>[12x]MGSSHHHHHHSQDLDEVDAGSMTEIVADKTVEVVKNAIETADGALDLYNKYLDQVIPWQTFDETIKELSRFKQEYSQAASVLVGDIKTLLMDSQDKYFEATQTVYEWCGVATQLLAAYILLFDEYNEKKASAQKDILIKVLDDGITKLNEAQKSLLVSSQSFNNASGKLLALDSQLTNDFSEKSSYFQSQVDKIRKEAYAGAAAGVVAGPFGLIISYSIAAGVVEGKLIPELKNKLKSVQNFFTTLSNTVKQANKDIDAAKLKLTTEIVAIGEIKTETETTRFYVDYDDLMLSLLKEAAKKMINTCNEYQKRHGKKTLFEVPEV

E. coli cytolysin A (ClyA), also known as hemolysin (HlyE) or silent hemolysin A (SheA), belongs to the α-PFT class. ClyA is a 34 kDa soluble monomer, containing mainly α-helices with only one β-tongue that transforms into α-helical elements in the pore complexes. Each protomer in the ClyA pore complexes is composed of five α-helices, namely αA1, αB, αC, αF, and αG. Here we report the cryo-EM structures of ClyA pore complexes in the presence of n-Dodecyl-β-D-Maltoside (DDM) as dodecamer, tridecamer, and tetradecamer at the resolution of 2.8 Å, 3.2 Å and 4.3 Å, respectively.

The crystal structure of the ClyA pore complex was previously solved as a dodecamer at 3.3 Å. The EM density map of the dodecamer presented here is at 2.8 Å, representing an improved density and structure model. One typical example is the side chain of Y196 from αF, which is buried in the membrane. With the cryo-EM density map, we were able to re-assign the side chain in parallel to, rather than pointing toward the hydrophobic membrane environment. One protomer from the dodecamer (Prot_12) was superimposed to a protomer from the crystal structure (Prot_cry). Based on the comparison, it is obvious that the binding of mercury atoms pushes away the C-terminus of the αG helix with a movement distance of 4.6 Å at the Cα of R291. This represents an artificial distortion of the local structure by heavy atoms, although the overall fold is not affected. Extensive hydrogen bonds and salt bridges, spanning from the transmembrane regions to the distal soluble regions, mediate the interaction between neighboring protomers within the dodecamer, which is also observed in the crystal structure. Based on the particle numbers of total particles and those used in final 3D reconstructions, the majority of the complexes were 12-meric, representing approximately 80% of all particles, while only 11% were 13-meric. The inner diameters near the extracellular edge of the pore are 70, 72 and 77 Å for the dodecamer, the tridecamer, and the tetradecamer, respectively.(2E)-3-[3-(3,5-dimethylphenyl)-2,1-benzoxazol-5-yl]prop-2-enoic 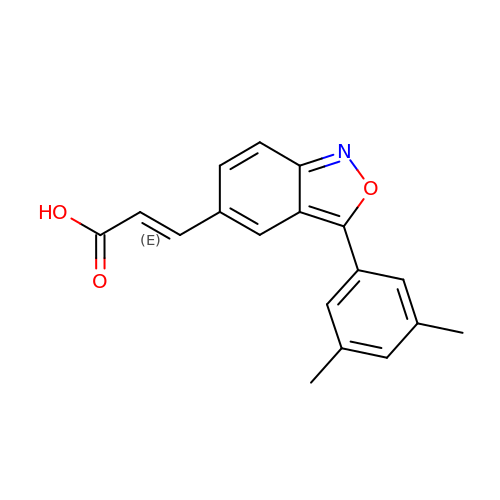acid | C18 H15 N O3 | GVBOPZONHGVWNG-GQCTYLIASA-N methyl N-(carboxymethyl)-N-(2-phenylethyl)glycyl-L-histidinate 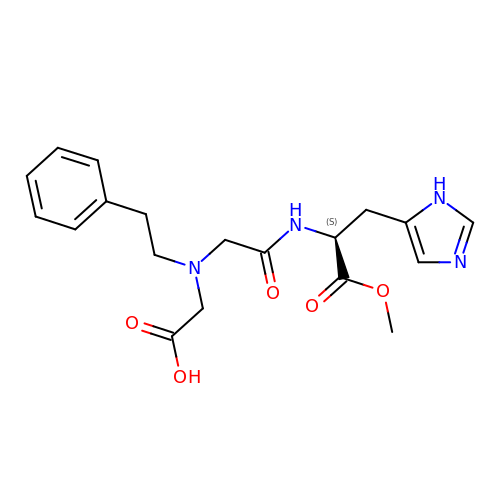| C19 H24 N4 O5 | GGPUXIJTYUPCEL-INIZCTEOSA-N(6S,9aS)-8-(anthracen-9-ylmethyl)-6-[(2S)-butan-2-yl]-4,7-bis(oxidanylidene)-N-[4,4,4-tris(fluoranyl)butyl]-3,6,9,9a-tetrahydro-2H-pyrazino[1,2-a]pyrimidine-1-carboxamide 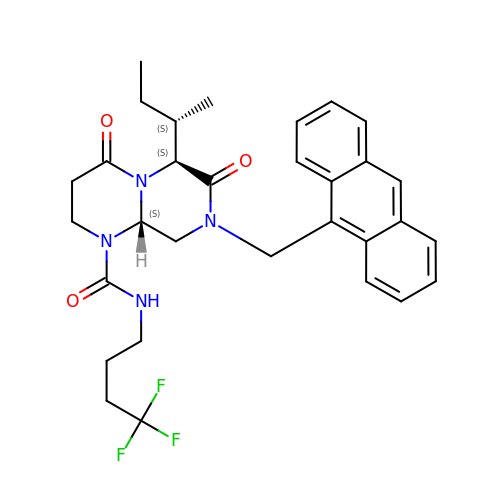| C31 H35 F3 N4 O3 | IPOJNTALVGAOOT-GFNGZDJJSA-N>GRSDAYTQVDNFLHAYARGGDELVNGHPSYTVDQAAEQILREQASWQKAPGDSVLTLSYSFLTKPNDFFNTPWKYVSDIYSLGKFSAFSAQQQAQAKLSLQSWSDVTNIHFVDAGQGDQGDLTFGNFSSSVGGAAFAFLPDVPDALKGQSWYLINSSYSANVNPANGNYGRQTLTHEIGHTLGLSHPGDYNAGEGDPTYADATYAEDTRAYSVMSYWEEQNTGQDFKGAYSSAPLLDDIAAIQKLYGANLTTRTGDTVYGFNSNTERDFYSATSSSSKLVFSVWDAGGN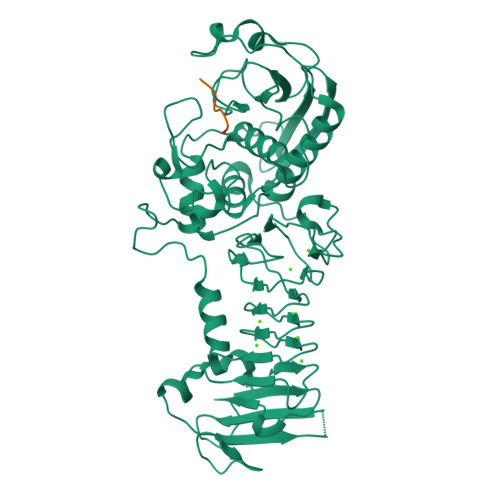DTLDFSGFSQNQKINLNEKALSDVGGLKGNVSIAAGVTVENAIGGSGSDLLIGNDVANVLKGGAGNDILYGGLGADQLWGGAGADTFVYGDIAESSAAAPDTLRDFVSGQDKIDLSGLDAFVNGGLVLQYVDAFAGKAGQAILSYDAASKAGSLAIDFSGDAHADFAINLIGQATQADIVV[2x];>[2x]RPKPQQ>METEIAKPLADFAYSLYQLEEAGNVFFSPVSIFLALAMVFFGSNGNTNTQLLNVMFKAGWKKNRTKKAMRSFVSSLTIDEYYDASLKLANRLYANDQYPILHPFLKDVKRYLSSDLVSVNFADTEAARLQINKWVSDQTNHKINDLLQSGTVEANTRLIAVNAIYFKASWDEVFDEAHTKPKKFYPTPHSSIKIPMMTQTNGYSYYETEDYQFLGMDYYPEYLKMFILLPKSGKTLSELQQKFNGETLLNLVSKVSGAEVKVTIPKMKFEKQMNLVEALKKLGIEDLFIPGKADLSGICVKEKLYVSDIVHKAYLEFNEEGTEAAAATAVRIVPMSGVMYEDSFEFVADHPFLFFIFDSRSKA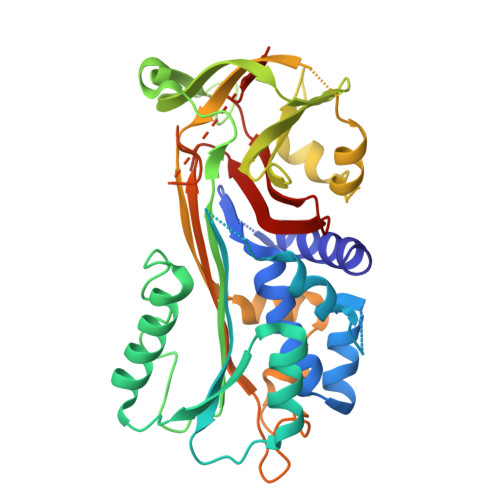ILFIGRFSGN[2x]(2R,4S)-2-[(1R)-1-{[(2'-carboxybiphenyl-2-yl)carbonyl]amino}-2-oxoethyl]-5,5-dimethyl-1,3-thiazolidine-4-carboxylic 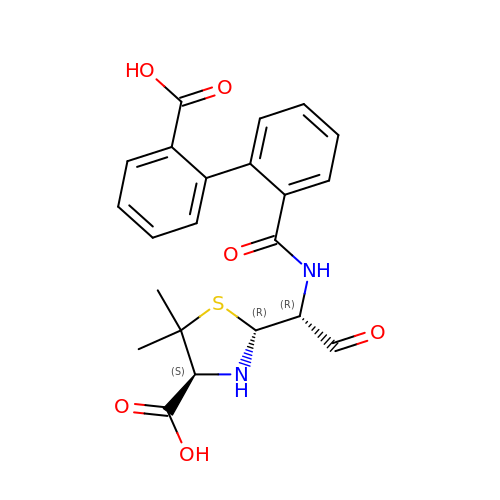acid | C22 H22 N2 O6 S | RFZQTRAFQUXQJP-ZIFCJYIRSA-N> SMMSDLHIPGTQSTPAIQGDWQAGRLSMQGDSYPENSYELFGQVIDWVERFLADGQRPLELDLRLLYLNTSSIKAMMDILDLLEEAHQGGRPVSLRWHYDRRNERVAELAEEFREDCSFPFAIQAHDE

Here, we show that the SiaABCD proteins play a key role in cellular aggregation and dispersal of P. aeruginosa in response to carbon availability in the environment. With our study, we demonstrated that the protein phosphatase SiaA and its kinase counterpart SiaB target the protein SiaC at threonine 68 (T68) and provide evidence that the SiaABC proteins make use of a partner switch mechanism to balance cellular aggregation in response to carbon availability. A partner switch system (PSS) typically involves a PP2C phosphatase (SiaA), an anti-sigma factor with kinase activity (SiaB) and anti-sigma factor antagonist representing the target for phosphorylation (SiaC). As such, that study is complementary to our data and strongly supports a model that the SiaABC partner switch integrates environmental information, such as carbon availability and surfactant stress, to control biofilm formation through the modulation the activity of SiaD through the phosphorylation status of SiaC.

To gain insights about SiaC, its crystal structure was determined in this study. Native crystals of SiaC were grown in C6 condition of the JCSG+ kit from Molecular Dimensions (0.1 M Phosphate/citrate, pH 4.2, 40% (v/v) PEG 300), with space group I222 and diffracted to a maximum resolution of 1.7 Å. Clear electron density maps allowed complete tracing except for residues 101–103, which are located in the flexible loop between the α3 helix and β5 strands. The SiaC protein comprises six β-strands arranged in a mixed parallel/antiparallel fashion and three α-helices. Notably, SiaC contains a putative phosphorylation site at threonine residue 68 (T68) and as such could represent the target of the predicted protein phosphatase/kinase activities of SiaA and SiaB. A hydrophobic pocket next to T68 is formed by residues L61 and L63 projecting from β4, W95 from β5, I71 and M74 from α2, L107 and F111 from α3 while L66 belongs to the β4-β5 loop. The hydrophobic pocket next to the phosphorylation site of SiaC is of particular interest, as it seems to be involved in the stability of the SiaA/SiaCP interaction. In addition, a large patch of negatively charged surface is present at α2 and α3 near the hydrophobic pocket, and could thus be useful for drug design as potential anchor points. In addition to SiaA inhibition, SiaC also represents an exciting target for interference, as it is structurally most similar to bacterial anti-sigma factor antagonists with little homology with human proteins.> CDNDTEPGGTAVEKMAGDWWVTVNAFIDGKEVEDPFGAGHLQMSTYNTASNSETEMWLDDLGNFWEYKLKVNVNYAARTFSTTGFVDNVTYESKVKITDGKVLEKAATTPSGMPADSI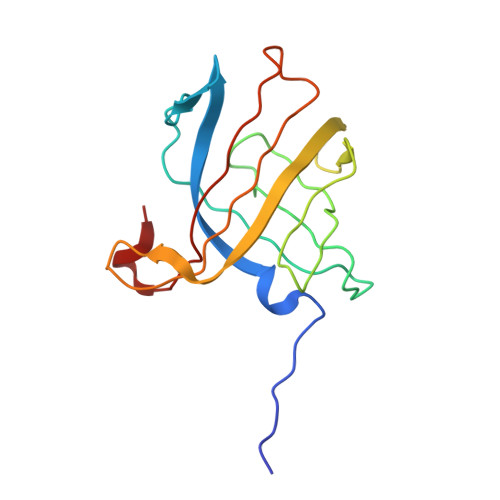VYMVQFDDDEDGLTYKVSGFRRTGFPADDF>[4x]HMSVNKVTCLVCRKGDND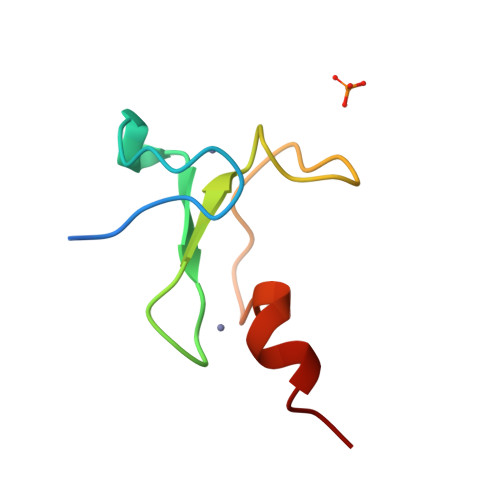EFLLLCDGCDRGCHIYCHRPKMEAVPEGDWFCTVCLAQQV>MNTVRSEKDSMGAIDVPADKLWGAQTQRSLEHFRISTEKMPTSLIHALALTKRAAAKVNEDLGLLSEEKASAIRQAADEVLAGQHDDEFPLAIWQTGSGTQSNMNMNEVLANRASELLGGVRGMERKVNPNDDVNKSQSSNDVFPTAMHVAALLALRKQLIPQLKTLTQTLNEKSRAFADIVKIGRTHLQDATPLTLGQEISGWVAMLEHNLKHIEYSLPHVAELALGGTAVGTGLNTHPEYARRVADELAVITCAPFVTA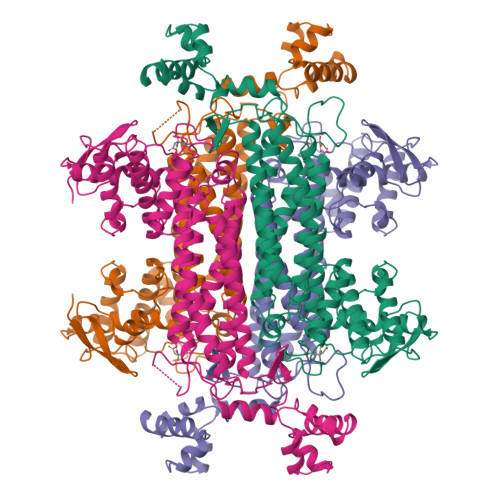PNKFEALATCDALVQAHGALKGLAASLMKIANDVRWLASGPRCGIGEISIPENEPGSSIMPGKVNPTQCEALTMLCCQVMGNDVAINMGGASGNFELNVFRPMVIHNFLQSVRLLADGMESFNKHCAVGIEPNRERINQLLNESLMLVTALNTHIGYDKAAEIAKKAHKEGLTLKAAALALGYLSEAEFDSWVRPEQMVGSMKAGR[2x]>HHHHHHTGLDLGAASSFGALAPQGVANAGATVINGDMGTTGTSITGFPPGLITGQLHINDDTSTQAFADSRTAFVAGQALIATVDQAGTATLGGNTFVAGVYKYDSAVGLDGVLTLDGAGDASSVW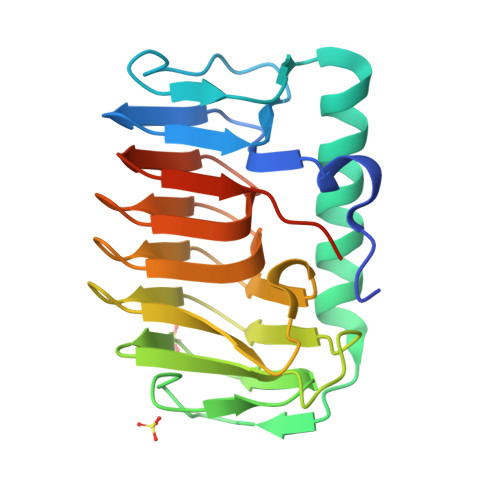VFQLATTLVTYASSSIILTNGAKANNVFWIVGSSATLGTYSHLEGNVIANALIAAQTGATINGALLAGSAVTLDSNTVTVQNSASKLVRSAKFFKV[6x]Non-ribosomal peptide synthetases (NRPS) are multi-modular/domain enzymes that catalyze the synthesis of bioactive peptides. A crucial step in the process is peptide elongation accomplished by the condensation (C) domain with the aid of a peptidyl carrier or thiolation (T) domain. Here, we examined condensation reaction carried out by NRPS AmbB involved in biosynthesis of l-2-amino-4-methoxy-trans-3-butenoic acid (AMB) in P. aeruginosa. We determined crystal structures of the truncated T–C bidomain of AmbB in three forms, the apo enzyme with disordered T domain, the holo form with serine linked phosphopantetheine (Ppant) and a holo form with substrate (l-alanine) loaded onto Ppant.

The Ppant transferase, Sfp enzyme, was used to convert the apo form of AmbB T–C into its holo state. Each of the two holo crystal structures have four T-C didomains in their asymmetric units. The Ppant arm is covalently tethered to the invariant Ser768 in the conserved GGXS motif, situated at the start of helix α2 of the T domain. The orientation of the T domain, places Ser768 at the donor entry side of the C domain of AmbB, with the Ppant arm extending into the donor pocket towards the active site. Among the four protomers in the structures of holo AmbB T-C tethered with Ppant, only protomer D shows well defined electron density for Ppant but the ligand is in an unproductive configuration, where the thiol moiety does not point towards the putative catalytic His953. Ppant resides in the donor pocket that leads to the catalytic groove of the C domain. At the entrance of the pocket, one of the two phosphate oxygen atoms of Ppant is hydrogen bonded to Ser1058 from the C domain. Leu769 and Phe1060 form a hydrophobic pocket around the gem dimethyl moiety of Ppant. The walls of the pocket lining the Ppant are constituted of Ala1085, Leu1086, Ala1087, Ala 1162 and Tryp 1194. The terminal thiol end of the Ppant is surrounded by Val1102, two negatively charged residues namely Asp957 and the highly conserved Asp958, as well as the catalytic His953.

>TGAEPQALPSDPLEQALHQAWQAQLGAPPRAGQGFYAAGGDSLRAVHLLATLRQRLSRRVPLQAFAGGPATPEALLELLRQAAPEGDEPEPSAGAAGLSLAERRLWVAQQLAPEDTSYNLLAHLRIVGATADAIEQALRQLLERHVALRRRVETGVDGPQPHALAAHAVPLQRLLASDAVHAERLLEDGVRREGARVFDLAHEAPARLLLVVTRDSARADLLLSVHHYAFDDVSLAVFAAELKTLLDGGRLGVLASTPEQVAARERAALASGRLDRVAERWAERLLPLAKAPGAAPARPEESGGRAGQRLALPVSAAVHAACRALAERTSVSPFSAALQAFAEVLGAELGVDDLLVGVALAGRSRLEMQGLVGCFVNLLPLAVGLRPEQSVEWRLRQVGHDLLELLEHQDVPLECVTQALRQRGASGLPIRIACGAHNGRAAPAVDAGVRVEADFIPVPGARLDLTLWLEDQPQGWLAVWTGVSAIFDLHRIERLHQAWERRLLANAGEPISKRMSPEGCNAS[4x]>XGEIAQALKEIAKAAAAALKEIAWALKEIAQALKGX[14x]

De novo coiled coils (CCs) are particularly appealing modules for designing self-assembling systems as they are short, mutable, and sequence-to-structure relationships governing their folding and assembly are well established. For example, CC-Tri and CC-Tet exchanged with each other, as did the higher-order CCs, CC-Pent2, CC-Hex2, and CC-Hept. These two classes—i.e., CC-Tri plus CC-Tet, and CC-Pent2, CC-Hex2 plus CC-Hept—are structurally distinct: the trimer and tetramer have consolidated hydrophobic cores, whilst the others have central channels and are α-helical barrels. Similarly, peptides with Type II interfaces where the g, a, d, and e residues all engage in helix–helix interactions—namely the pentameric, hexameric, and heptameric α-helical barrels, CC-Pent2, CC-Hex2 and CC-Hept—also exchange with each other. To address this, using the insight from the data and analysis presented here, we have tested two different strategies for increasing specificity of coiled coils: (i) alternate placement of salt bridge-promoting residues, lysine and glutamate to discriminate the tetramer from the trimer; and (ii) incorporation of hendecad repeats to separate the α-helical barrels.

For the α-helical barrels, CC-Pent2, CC-Hex2, and CC-Hept, designing orthogonal variants was more challenging. Therefore, we took a different approach of incorporating non-heptad sequence repeats into these peptide sequences. Variations of this 3-4 spacing can lead to alternative CC sequences and structures. For instance, in 11-amino acid, hendecad repeats core-forming residues are spaced 3-4-4 apart at the a, d, and h sites of a → k repeats (Fig. S38†).16,63–67 Consequently, while heptad repeats drive association of left-handed CCs, hendecads lead to right-handed quaternary structures (Fig. S38†).16,63–67 We reasoned that replacing heptad with hendecad repeats at different locations in the pentamer, hexamer, and heptamer sequences should alter the hydrophobic seams and, in turn, might confer homo-specificity in the resulting sequences. Initially, we made several variants of CC-Pent2, CC-Hex2, and CC-Hept that extended the second heptads into hendecad repeats, with the new designs denoted by the suffix “-hen2”. In these, the original a-g sequences were maintained, and the new i-k sites were all made Ala. So, we tested Ala, Ile, and Leu in each of the three designs. Generally, for the CC-Pent2 and CC-Hept designs, these experiments revealed less exchange between the heptad and hendecad variants compared to the homotypic exchange of the parents, indicating that the strategy had increased orthogonality. To investigate this and test our hypothesis of altering the hydrophobic seams, we compared model and experimental structures of CC-Pent2-hen2, CC-Hex2-hen2, and CC-Hept-hen2 with Ala at the h position.> VTTKQWMSALPDTTNLAALSIPGTHDTMSYNGDITWTLTKPLAQTQTMSLYQQLEAGIRYIDIRAKDNLNIYHGPIFLNASLSGVLETITQFLKKNPKETIIMRLKDEQNSNDSFDYRIQPLINIYKDYFYTTPRTDTSNKIPTLKDVRGKILLLSENHTKKPLVIN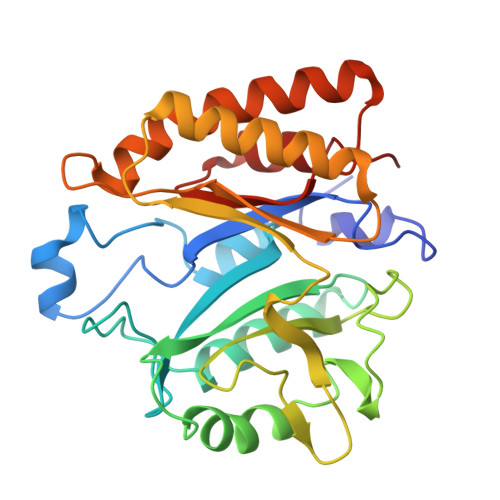SRKFGMQFGAPNQVIQDDYNGPSVKTKFKEIVQTAYQASKADNKLFLNHISATSLTFTPRQYAAALNNKVEQFVLNLTSEKVRGLGILIMDFPEKQTIKNIIKNNKF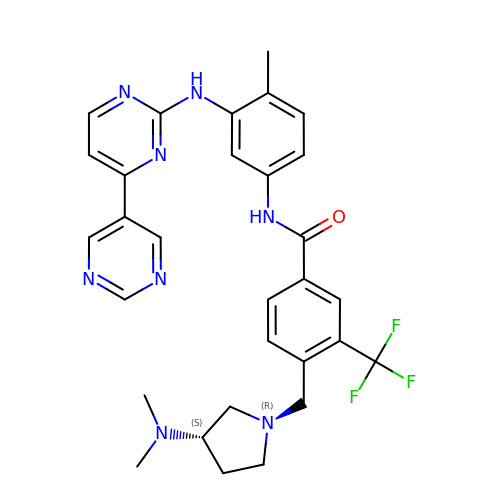N-[3-(4,5'-BIPYRIMIDIN-2-YLAMINO)-4-METHYLPHENYL]-4-{[(3S)-3-(DIMETHYLAMINO)PYRROLIDIN-1-YL]METHYL}-3-(TRIFLUOROMETHYL)BENZAMIDE | C30 H31 F3 N8 O | ZGBAJMQHJDFTQJ-DEOSSOPVSA-N>SDALKVRWPDFNQEAYVGGTMVRSGQDPYARNKFNQVESDKLRMDRAIPDTRHDQCQRKQWRVDLPATSVVITFHNEARSALLRTVVSVLKKSPPHLIKEIILVDDYSNDPEDGALLGKIEKVRVLRNDRREGLMRSRVRGADAAQAKVLTFLDSHCECNEHWLEPLLERVAEDRTRVVSPIIDVINMDNFQYVGASADLKGGFDWNLVFKWDYMTPEQRRSRQGNPVAPIKTPMIAGGLFVMDKFYFEELGKYDMMMDVWGGENLEISFRVWQCGGSLEIIPCSRVGHVFRKQHPYTFPGGSGTVFARNTRRAAEVWMDEYKNFYYAAVPSARNVPYGNIQSRLELRKKL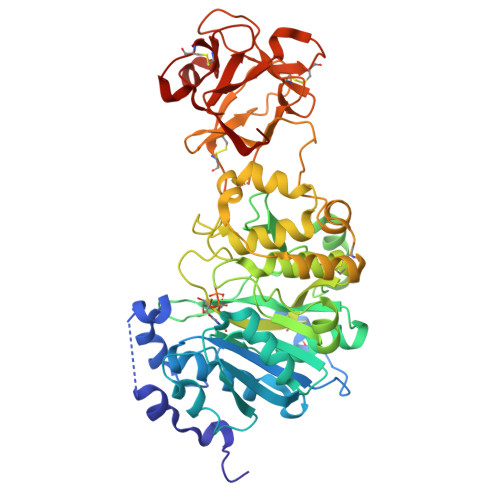SCKPFKWYLENVYPELRVPDHQDIAFGALQQGTNCLDTLGHFADGVVGVYECHNAGGNQEWALTKEKSVKHMDLCLTVVDRAPGSLIKLQGCRENDSRQKWEQIEGNSKLRHVGSNLCLDSRTAKSGGLSVEVCGPALSQQWKFTLNLQQ[2x]> ASTLKSGSKEVENLKKPFMPPREVHVQVTHSMPPQKIEIFKSLDNWAEENILVHLKPVEKCWQPQDFLPDPASDGFDEQVRELRERAKEIPDDYFVVLVGDMITEEALPTYQTMLNTLDGVRDETGASPTSWAIWTRAWTAEENRHGDLLNKYLYLSGRVDMRQIEKTIQYLIGSGMDPRTENSPYLGFIYTSFQERATFISHGNTARQ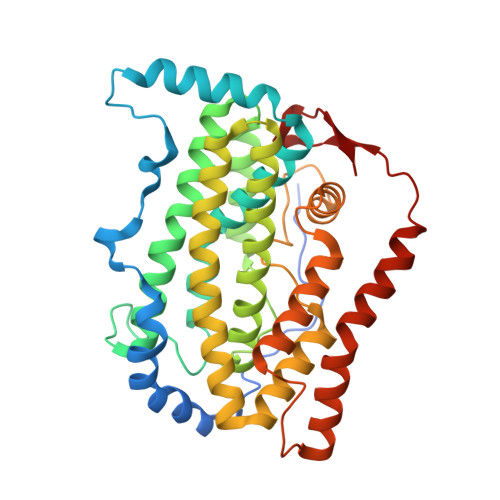AKEHGDIKLAQICGTIAADEKRHETAYTKIVEKLFEIDPDGTVLAFADMMRKKISMPAHLMYDGRDDNLFDHFSAVAQRLGVYTAKDYADILEFLVGRWKVDKLTGLSAEGQKAQDYVCRLPPRIRRLEERAQGRAKEAPTMPFSWIFDRQVKL> QSRAIMDYQDRVTHMDENDYKKIINRAKEYNKQFKTSGMKWHMTSQERLDYNSQLAIDKTGNMGYISIPKINIKLPLYHGTSEKVLQTSIGHLEGSSLPIGGDSTHSILSGHRGLPSSRLFSDLDKLKVGDHWT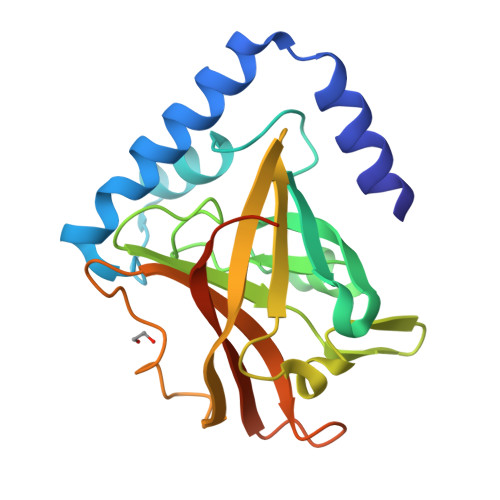VSILNETYTYQVDQIRTVKPDDLRDLQIVKGKDYQTLVTCTPYGVNTHRLLVRGHRVPNDNGNALVVAEAIQIE>[4x]MAT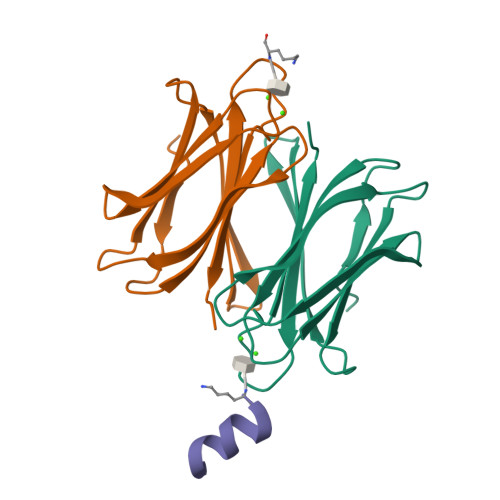QGVFTLPANTRFGVTAFANSSGTQTVNVLVNNETAATFSGQSTNNAVIGTQVLNSGSSGKVQVQVSVNGRPSDLVSAQVILTNELNFALVGSEDGTDNDYNDAVVVINWPLG;>KKLLKLLKLLLX[4x]> GPSKQPDLKKMEQESIDQLCELKKLKQFDIQPDGHSLFASILDQLKLRHDPKKLDQDMDVMKLRWLSCNYVQEHRDDFIPYL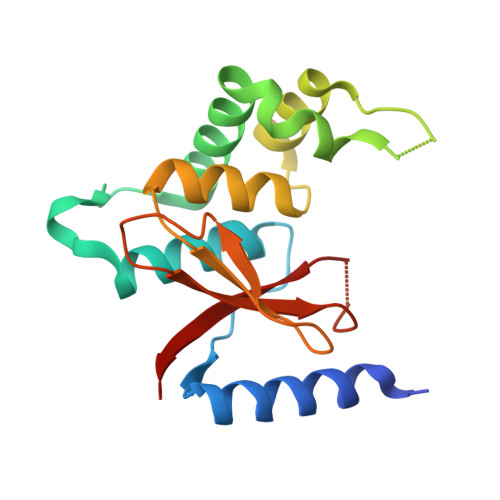FDEETMKMKDIDEYTKEMEHTAQWGGEIEILALSHVFDCPISILMSGRPIQVYNECGKNPELKLVYYKHSYALGEHYNSLHDS> SSSQRMEHILICCVCLGDNSEDADEIIQCDNCGVTVHEGCYGVDGESDSIMSSASENSTEPWFCDACKNGVSPSCELCPSQDGIFKETDAGRWVHVVCALYVPGVAFGDIDKLRPVTLTEMNYSKYGAKECSLCEDTRFARTGVCISCDAGMCRSFFHVTCAQREGL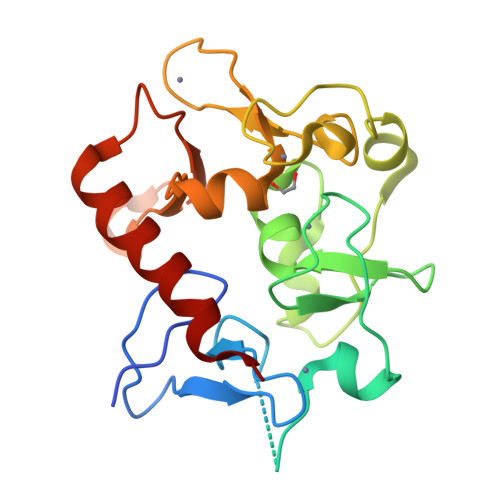LSEAAAEEDIADPFFAYCKQHADRFDRKWKRKNYLALQSYCKVS> MGHHHHHHENLYFQGMKKEKVEQILAEFQLQEEDLKKVMRRMQKEMDRGLRLETHEEASVKMLPTYVRSTPEGSEVGDFLSLDLGGTNFRVMLVKVGEGEEGQWSVKTKHQMYSIPEDAMTGTAEMLFDYISECISDFLDKHQMKHKKLPLGFTFSFPVRHEDIDKGILLNWTKGFKASGAEGNNVVGLLR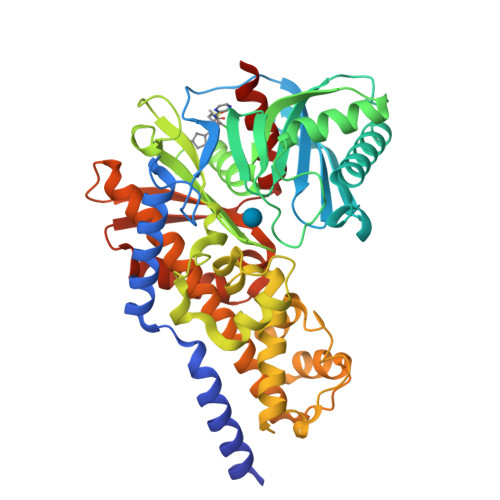DAIKRRGDFEMDVVAMVNDTVATMISCYYEDHQCEVGMIVGTGCNACYMEEMQNVELVEGDEGRMCVNTEWGAFGDSGELDEFLLEYDRLVDESSANPGQQLYEKLIGGKYMGELVRLVLLRLVDENLLFHGEASEQLRTRGAFETRFVSQVESDTGDRKQIYNILSTLGLRPSTTDCDIVRRACESVSTRAAHMCSAGLAGVINRMRESRSEDVMRITVGVDGSVYKLHPSFKERFHASVRRLTPSCEITFIESEEGSGRGAALVSAVACKKACMLGQ> MDLNLNRADYLQVGVTSQKTMKLLPASKHRATQKVVVGDHDGIVMCFGMKKGEAVTVFKTLPGQKIARLELGGALNTPQEKIFIAAGSEIRGFTKRGKQFLSFETNLTESIKAMHISGSDLFLSASYIYNHYCDCKDQHYYLSGDKINDVICLPVERLLREVPVLACQDRVLRVLQGSDVTYEIEVPGPPTVLALHNGNGGDSGEDLLFGTSDGKLGLIQITTSKPIHKWEIRNEKKRGGILCVDSFDIVGDGVKDLLVGRDDGMVEVYGFDNANEPVLRFDHTLSES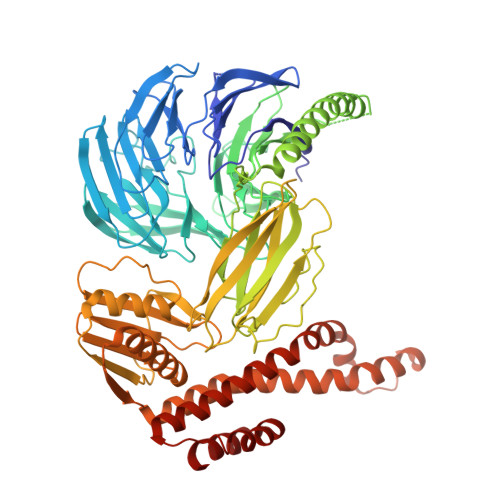VTSIQGGCVGKDGYDEIVVSTYSGWITGLTTEPVHKESGPGEELKFNQEMQNKISSLRSELEQLQYKVLQEREKYQQSSQSSKAKSAVPSFSVNDKFTLNKDDASYSLILEVQTAIDNVLIQSDVPIDLLDVDKNSAVVSFSSCDSESNDNFLLATYRCQANTTRLELKIRSIEGQYGTLQAYVTPRIQPKTCQVRQYHIKPLSLHQRTHFIDHDRPMNTLTLTGQFSFSELHSWVVFCMPEVPEKPPAGECVTFYFQNTFLDTQLESTYRKGEGVFKSDNISTISILKDVLSKEATKRKINLNISYEINEVSVKHTLKLIHPKLEYQLLLAKKVQLIDALKELQVHEGNTNFLIPEYRCILEEADHLQEEYKKQPAHLERLYGMITDLFIDKFKFKGTNVKTKVPLLLEILDSYDQNALIAFFDAA> GSHMASMTGGQQMGRDP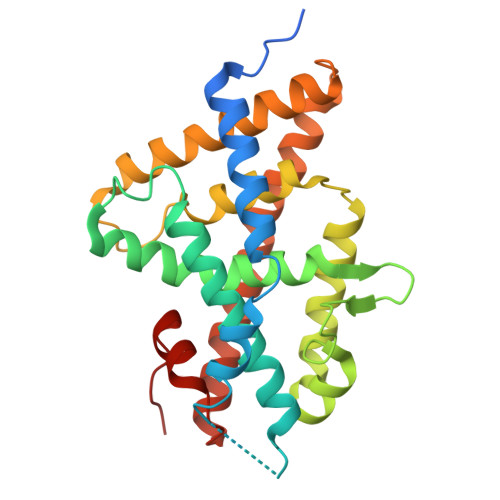LKNVPPLTANQKSLIARLVYYQEGYEQPSEEDLKRVTQTWQSDEDDEDSDMPFRQITEMTILTVQLIVEFAKGLPGFSKISQSDQITLLKACSSEVMMLRVARRYDAATDSVLFANNQAYTRDNYRKAGMAYVIEDLLHFCRCMYSMMMDNVHYALLTAIVIFSDRPGLEQPSLVEEIQRYYLNTLRVYILNQNSASPRSAVIFGKILGILTEIRTLGMQNSNMCISLKLKNRKLPPFLEEIWDVADVA>[4x]AEKPKLHYFNARGRMESTRWLLAAAGVEFEEKFIKS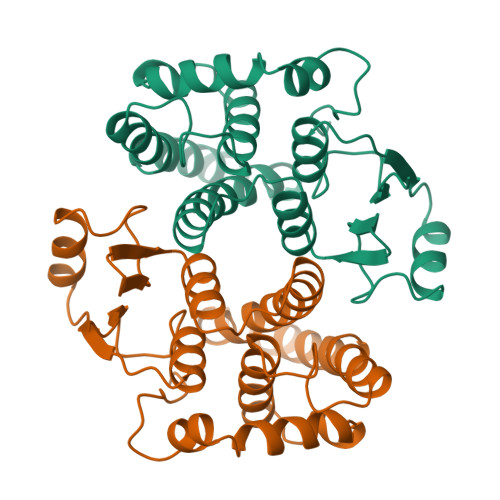AEDLDKLRNDGYLMFQQVPMVEIDGMKLVQTRAILNYIASKYNLYGKDIKERALIDMYIEGIADLGEMILLLPVCPPEEKDAKLALIKEKIKNRYFPAFEKVLKSHGQDYLVGNKLSRADIHLVELLYYVEELDSSLISSFPLLKALKTRISNLPTVKKFLQPGSPRKPPMDEKSLEEARKIFRF>HHHHHHMSAIKPDMKINLRMEGNVNGHHFVIDGDGTGKPFEGKQSMDLEVKEGGPLPFAFDILTTAFHYGNRVFAEYPDHIQDYFKQSFPKGYSWERSLTFEDGGICIARNDITMEGDTFYNKVRFHGVNFPANGPVMQKKTLKWEPSTEKMYVRDGVLTGDITMALLLEGNAHYRCDSRTTYKAKEKGV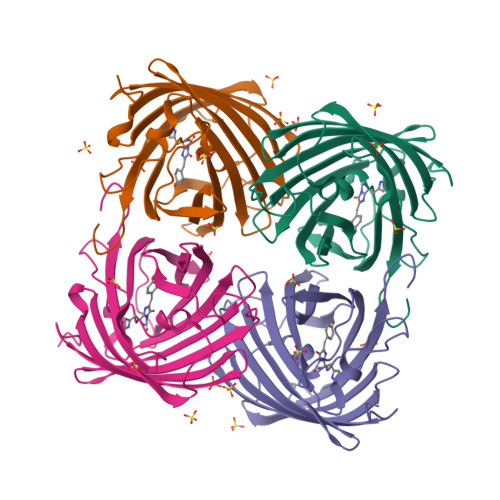KLPGYHLVDHCIEILSHDKDYNKVKLYEHAVAHSGLPDNARR[4x]>[5x]GSHMGGVEVLEVKTGVDSITEVECFLTPEMGDPDEHLRGFSKSISISDTFESDSPNRDMLPCYSVARIPLPNLNEDLTCGNILMWEAVTLKTEVIGVTSLMNVHSNGQATHDNGAGKPVQGTSFHFFSVGG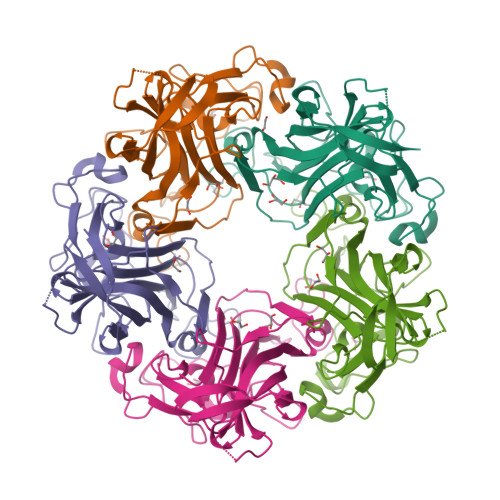EALELQGVLFNYRTKYPDGTIFPKNATVQSQVMNTEHKAYLDKNKAYPVECWVPDPTRNENTRYFGTLTGGEWVPPVLHITNTATTVLLDEFGVGPLCKGDNLYLSAVDVCGMFTNRSGSQQWRGLSRYFKVQLRKRRVKN Succinic semialdehyde dehydrogenase (SSADH) belongs to the aldehyde dehydrogenases (ALDH) superfamily and has been identified and purified from mammals as well as from microorganisms. SSA is then converted to succinic acid (SA) by the NAD+/NADP+-dependant enzyme succinic semialdehyde dehydrogenase (SSADH; EC 1.2.1.24). In Escherichia coli, two genetically distinct forms of SSADHs had been described that are essential for preventing accumulation of toxic levels of succinic semialdehyde (SSA) in cells. The gabD gene encodes a NADP+ dependent SSADH (EC 1.2.1.24) and is located in the gab operon.

In the present study, we begin to address this problem by determining the 2.3 Å X-ray crystal structure of SSADH from E. coli. The structure of E. coli SSADH reveals four monomers (A–D, 481 amino acid per monomer) in the asymmetric unit, forming, like other members of the aldehyde dehydrogenase (ALDH) family, a biologically relevant homotetramer with the 4 monomers related by a non-crystallographic 222 symmetry. The L-shaped molecule consists of three domains: The catalytic domain (residues 256–439), the cofactor binding domain (1–124, 146–254 and 446–471) and the oligomerisation domain (residues 125–147, 472–481). In each monomer, the cofactor NADP+ is bound to the active site giving rise to a binary complex, whereas the structure of the N-terminal His-tag was not resolved. E. coli SSADH was crystallised in the presence of both NADP+ and SSA. We observe no electron density for the substrate. Importantly our structural data permits unambiguous placement of the entire NADP+ moiety including that of the nicotinamide ring in each active site. In our structure, the NO2 and NO3 of the nicotinamide ribose interacts with E385 and K338 respectively; while NO7 of the nicotinamide ring binds to the backbone of L255 and G232 of the catalytic domain. A key difference between these two enzymes is that human SSADH utilizes NAD+ as a cofactor, whereas E. coli SSADH utilizes NADP+. Our structural data reveals the basis for this preference - in E. coli SSADH a three-residue deletion (of the human sequence 261RKN263) in the loop connecting s5C and h6 permits accommodation of the extra phosphate group of NADP+ (2'phosphate: Figure 3B, 4A and B). Significantly, our results show that E. coli gabD gene product is inactive in the presence of H2O2 and can be reactivated upon addition of DTT.

>KLNDSNLFRQQALINGEWLDANNGEAIDVTNPANGDKLGSVPKMGADETRAAIDAANRALPAWRALTAKERATILRNWFNLMMEHQDDLARLMTLEQGKPLAEAKGEISYAASFIEWFAEEGKRIYGDTIPGHQADKRLIVIKQPIGVTAAITPWNFPAAMITRKAGPALAAGCTMVLKPASQTPFSALALAELAIRAGVPAGVFNVVTGSAGAVGNELTSNPLVRKLSFTGSTEIGRQLMEQCAKDIKKVSLELGGNAPFIVFDDADLDKAVEGALASKFRNAGQTCVCANRLYVQDGVYDRFAEKLQQAMSKLHIGDGLDNGVTIGPLIDEKAVAKVEEHIADALEKGARVVCGGKAHERGGNFFQPTILVDVPANAKVSKEETFGPLAPLFRFKDEADVIAQANDTEFGLAAYFYARDLSRVFRVGEALEYGIVGINTGIISNEVAPFGGIKASGLGREGSKYGIEDYLEIKYMCIGL[4x]>[3x]GADNNKWKPLFGKNLENANYNPEVWSETDGVLGAVKD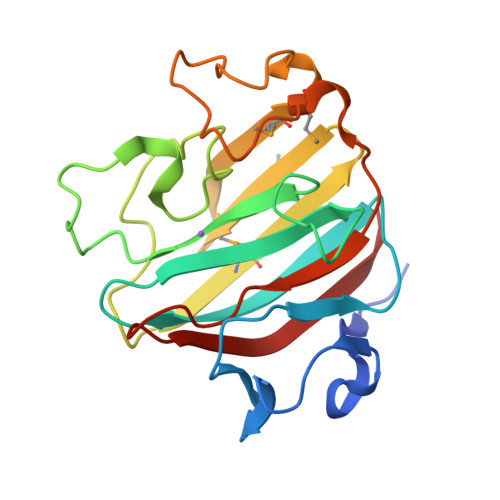ESIWTKDEYENFELDLDFKTDVGTNSGVVVYCTDTKDWIPNSVEIQIADDHCEKWGNGKPYEKCGAIYGHLGAVQDKVVKKPGEWNHMRIKCAGQHIMVILNGKKVTEMDMSKWTSGTKNPDGSDIPSWLPKPFAELPTKGFIGLQGKHGDSLIWFRNIKIRSL> MTDRYEQINDYIEALLKPRPDNVKRLEAYAEEHHVPIMEKAGMEVLLQILSVKQPKKILEIGTAIGYSAIRMALELPSAEIYTIERNEKRHEEAVNNIKEFQLDDRIHVFYGDALELADAVHVTAPYDVIFIDAAKGQYQNFFHLYEPMLSPDGVIITDNVLFK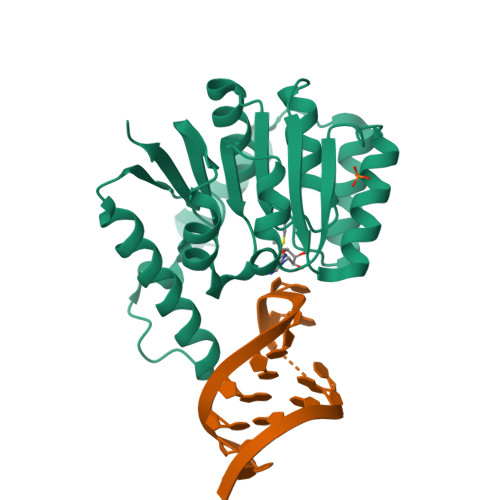GLVAEDYSKIEPKRRRRLVAKIDEYNHWLMNHPDYQTAIIPVGDGLAISKKKRGHHHHHHG> GSHMIYKEEGQEYAQITKMLGNGRVEASCFDGNKRMAHIRGKLRKKVWMGQGDIILVSLRDFQDDQCDVVHKYNLDEARTLKNQGELPENAKINETDNFGFESDEDVNFEFGNADEDD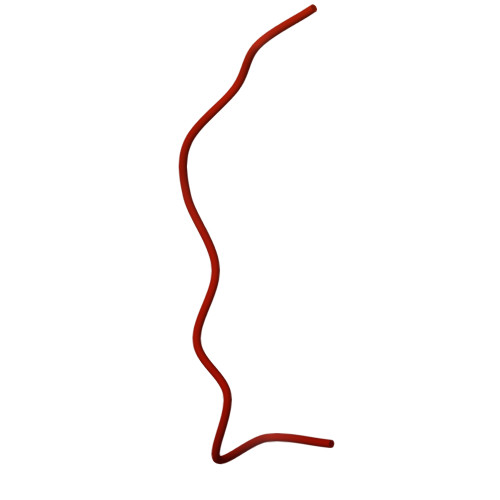EEGEDEELDIDDI> SLSEQALNHEKLMRAIVKNLADTPMVLKGETALYLGYGLNRFSEDLDFDCHKKINLLGRVKSAIPNGIILNDIHIKKDTDSVGRYMVRYATKDNKEEQTLKLEISYRDAPKESEVNVIEGMRIAKIERIIDNKLCACFDGEHTRTKARDLFDLHFLAKHYEEHFNLDLASRLKDFSKDPDKLVSDYLVDVKLDALLNQIMDLEETALELGVMAQLIHKKLEKQSHSLNALQE

JHP933, a conserved putative protein of unknown function, is encoded by the gene in plasticity region of H. pylori strain J99. Our work demonstrates that JHP933 is a nucleotidyltransferase superfamily protein with a characteristic αβαβαβα topology. Most NTase fold proteins can transfer nucleoside monophosphate (NMP) from substrate nucleoside triphosphate (NTP) to the hydroxyl group of their second substrate, such as a small molecule, nucleic acid or protein. The molecular details regarding the function of JHP933 are unknown due to the lack of sequence similarity with other well-characterized proteins.

The final crystal structure of JHP933, containing residues 11–243, was refined at a resolution of 2.1 Å with a Rwork and Rfree of 20.43% and 23.08%, respectively. The overall structure of JHP933 consists of two domains: an N-terminal core domain and a C-terminal tail domain. The N-terminal core domain covers residues 11–170 and contains 5 α-helices (α1–α5) and 7 β-strands (β1–β7). The C-terminal tail domain is formed by α-helices α6–α7 followed by an extended α-helix (α8). The N-terminal core domain of JHP933 has an αβαβαβα topology formed by α1-β1-α2-β2-α3-β5-α4, which is coincident with the common α/β-fold structure of nucleotidyltansferase (NTase) fold proteins. A Dali search for structural homology identified lincosamide antibiotic adenylyltransferase LinA as the closest related structure with a Z-score of 9.6. By comparison to the active site of LinA complex structure, a conservative large cleft is identified as a possible active site for substrate binding at the N-terminal core domain of JHP933. This substrate-binding cleft is surrounded mainly by β-strands β1, β2, β5 and α-helices α4, α2 with a size of around 13×20×20 Å. The corresponding residues are G39, D55hD57 and E113 in JHP933; with G39 at the connection of β1 and α2, D55 and D57 located on β2, and E113 is placed on β5 structurally adjacent to β2. Therefore, with reference to the structural conservation of these NTase superfamily proteins, the conserved G39 should play a crucial role in binding of substrates, and D55/D57 and E113 likely are involved in the coordination of divalent ions such as Mg2+, which chelates the phosphates of a nucleoside triphosphate substrate and plays a crucial role in activation of the second substrate's hydroxyl group.> GSHMPAGAGQDGRRIARIE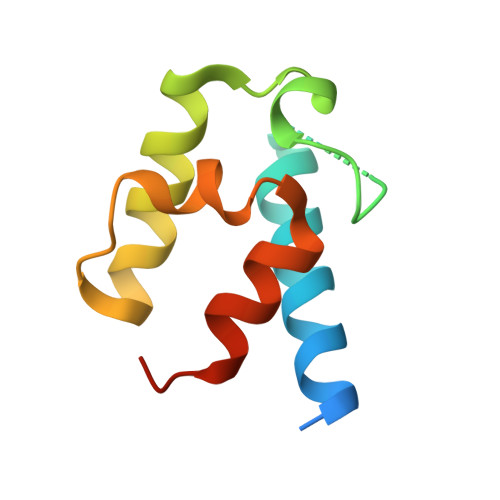EDLRRLVSARIEAPSQAVDAEESFFSLGVDSVALQEITETLERTYGSLPPTLLFENPNIRQLARYLAERVPARSA>GEVANPEHYIKHPLQNRWALWFFKNDKSKTWQANLRLISKFDTVEDFWALYNHIQLSSNLMPGCDYSLFKDGIEPMWEDEKNKRGGRWLITLNKQQRRSDLDRFWLETLLCLIGESFDDYSDDVCGAVVNVRAKGDKIAIWTTECENRDAVTHIGRVYKERLGLPPKIVIGYQSHADTATKSGSTTKNRFVV[2x];>[2x]GEFST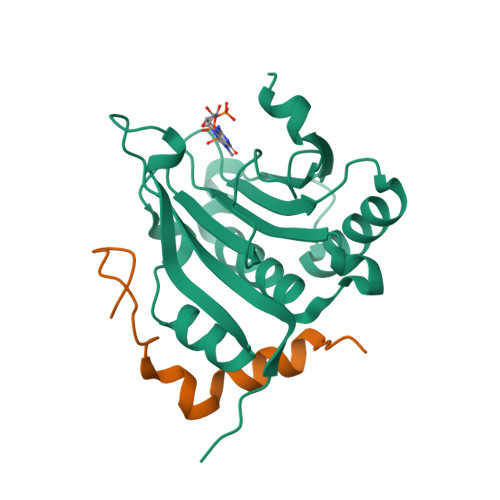TPGGTRIIYDRKFLMECRNSPVTKTPPRDLPTIPGVTSP> ISGGDAIYSSTGRCSLGFNVRSGSTYYFLTAGHCTDGATTWWANSARTTVLGTTSGSSFPNNDYGIVRYTNTTIPKDGTVGGQDITSAANATVGMAVTRRGSTTGTHSGSVTALNATVNYGGGDVVYGMIRTNVCAEPGDSGGPLYSGTRAIGLTSGGSGNCSSGGTTFFQPVTEALVAYGVSVY;> VD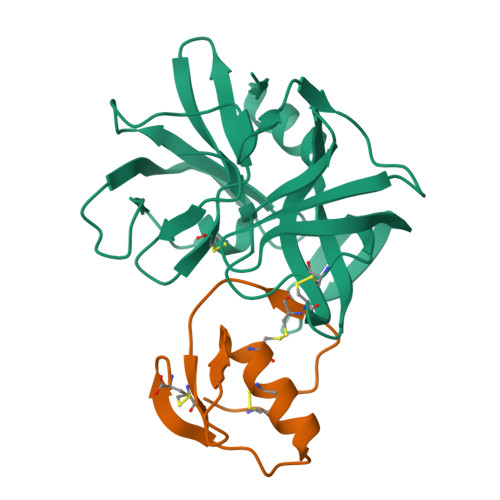CSEYPKPACTIEYRPLCGSDNKTYGNKCNFCNAVVESNGTLTLSHFGKC(2R)-1-{[(5-methylthiophen-2-yl)methyl]amino}propan-2-ol 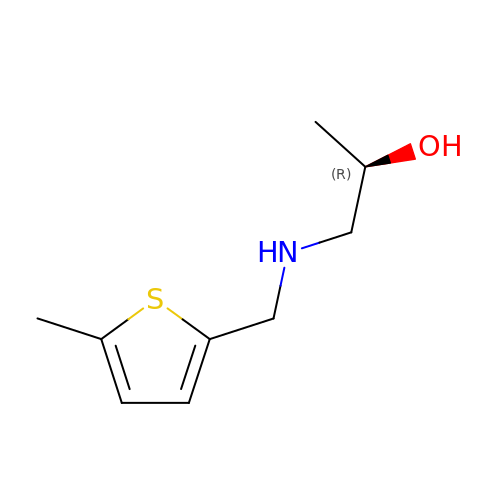| C9 H15 N O S | JLVFMHMDKADIAM-SSDOTTSWSA-N> TAG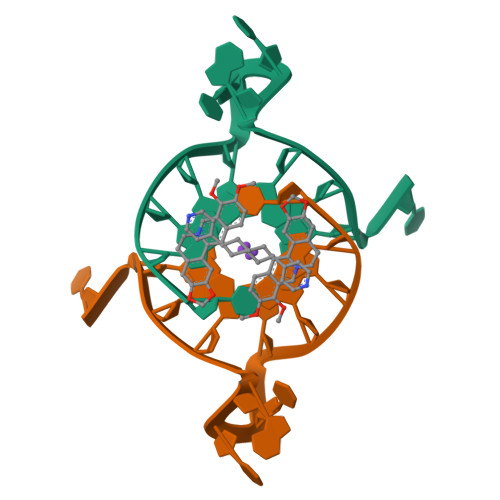GGTTAGGGT> GSPEFMDDIFTQCREGNAVAVRLWLDNTENDL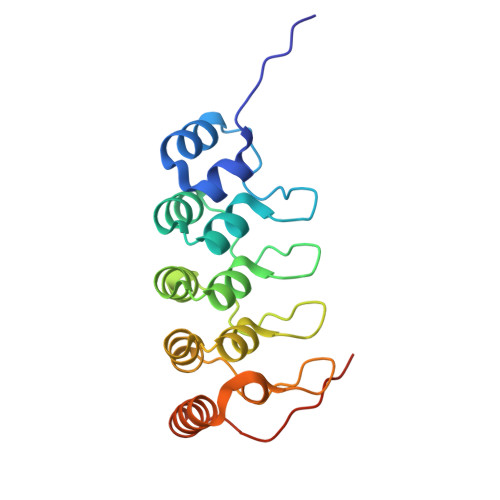NQGDDHGFSPLHWACREGRSAVVEMLIMRGARINVMNRGDDTPLHLAASHGHRDIVQKLLQYKADINAVNEHGNVPLHYACFWGQDQVAEDLVANGALVSICNKYGEMPVDKAKAPLRELLRERAEKMGQNLNRIPYKDTFWKGTTR> ALDI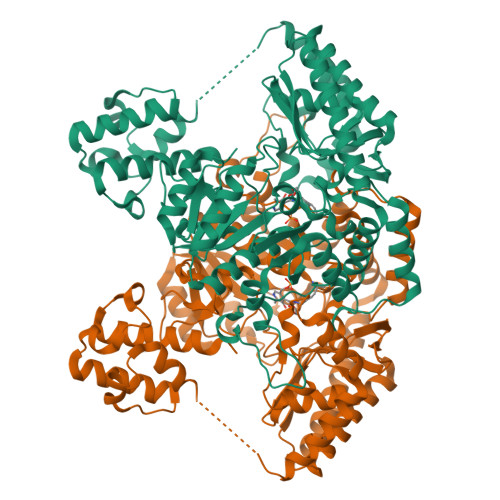NHTKTHIESFLKTVISNASGIRADEIDSNAHFIGFGLDSIMLTQVKKAIADEFNVDIPMERFFDTMNNIESVVDYLAENVPSAASGSLNEQVNYTPQQRQYLESFIEKYVDKTKGSKQYTDETRFAHANNRNLSSFRSYWKEMVYPIIAERSDGSRMWDIDGNEYIDITMGFGVNLFGHHPSFITQTVVDSTHSALPPLGPMSNVAGEVADRIRACTGVERVAFYNSGTEAVMVALRLARAATGRTKVVVFAGSYHGTFDGVLGVANTKGGAEPANPLAPGIPQSFMNDLIILHYNHPDSLDVIRNLGNELAAVLVEPVQSRRPDLQPESFLKELRAITQQSGTALIMDEIITGFRIGLGGAQEWFDIQADLVTYGKIIGGGQPLGIVAGKAEFMNTIDGGTWQYGDDSYPTDEAKRTFVAGTFNTHPLTMRMSLAVLRYLQAEGETLYERLNQKTTYLVDQLNSYFEQSQVPIRMVQFGSLFRFVSSVDNDLFFYHLNYKGVYVWEGRNCFLSTAHTSDDIAYIIQAVQETVKDLRRGGFIPEGPDS>GQDMVSPPPPIADEPLTVNTGIYLIECYSLDDKAQTFKVNAFLSLSWKDRRLAFDPVRSGVRVKTYEPEAIWIPEIRFVNVENARDADVVDISVSPDGTVQYLERFSARVLSPLDFRRYPFDSQTLHIYLIVRSVDTRNIVLAVDLEKVGKNDDVFLTGWDIESFTAVVKPANFALEDRLESKLDYQLRISRQYFSYIPNIILPMLFILFISWTAFWSTSYEANVTLVVSTLIAHIAFNILVETNLPKTPYMTYTGAIIFMIYLFYFVAVIEVTVQHYLKVESQPARAASITRASRIAFPVVFLLANIILAFLFFGF[5x]

At present, the best structurally characterized pLGIC is the G. violaceus ligand-gated ion channel (GLIC), of prokaryotic origin. Each subunit consists of an extracellular domain (ECD), predominantly in a β-sandwich fold, and a transmembrane domain (TMD) composed of four helices, labeled M1–M4. However, the GLIC is a pH-gated channel, activated by lowering the pH, with a maximal activation at pH 4 and a pH50 around 5. We instead found that proton activation is a complex multiple loci mechanism, with the key contribution stemming from the coupling interface between the extracellular and transmembrane domain, with E35 acting as a key proton-sensing residue.

Finally, mutation of E35 produced the strongest effect; therefore, a more extensive study of this position was performed. The mutations E35Q, E35A, and E35M (the GlyR-position equivalent) display a significant increase in pH50, whereas E35K shows a weaker nonsignificant effect, and E35H appears to show the inverse phenotype with a marked decrease in pH50. Altogether, these data show that the loss of charge at the E35 position is important to the gain-of-function effect found. Mutants of E35 are unique in strongly increasing the proton sensitivity. Neutralization of the E35 side chain by mutation to A, Q, or M produce a similar increase in proton sensitivity, whereas the mutation of E35K exhibits the same behavior with half the increase. Interestingly, the structures of the Wt GLIC, E35Q, and E35A at pH 4 show that the side chain of residue 35 is located in a hydrophobic environment bordered by the side chains of P113, L114, F116, F156, T158, and P247. In the GLIC structure at pH 7, which is representative of the resting state, the carboxyl moiety of E35 is more solvent exposed toward the inner vestibule because the side chain of P247 is moved away following the key revolving motion of the M2–M3 loop. Therefore, the resting state would be predicted to better accommodate a charged residue, which is consistent with the functional data. Altogether, the data support that E35 is a bona fide proton sensor, whose charged form stabilizes the resting conformation, whereupon protonation favors the active state. The functional proton gating of E35Q and E35A mutants additionally suggests that if E35 is a bona fide proton sensor, it can’t be the only one in the GLIC.>[2x]GAMGDSIKQLLM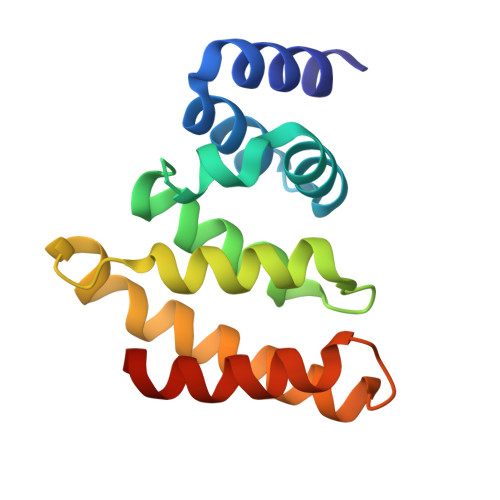AGQINKAFHQALLANDLGLVEFTLRHTDSNQAFAPEGCRLEQKVLLSLIQQISADMTNHNELKQRYLNEALLAINMADPITREHAPKVLTELYRNCQQFIKNSPKNSQFSNVRLLMKAIITYRDQLK> DPASNL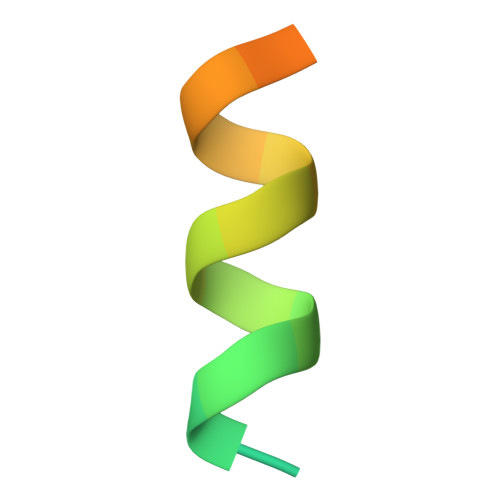GLEDIIRKALMGSFDDK>MGHHHHHHMKLTPELTPFVLFTGFEPVQVQQYIKKLYILGGEVAESAQKCTHLIASKVTRTVKFLTAISVVKHIVTPEWLEECFRCQKFIDEQNYILRDAEAEVLFSFSLEESLKRAHVSPLFKAKYFYITPGICPSLSTMKAIVECAGGKVLSKQPSFRKLMEHKQNSSLSEIILISCENDLHLCREYF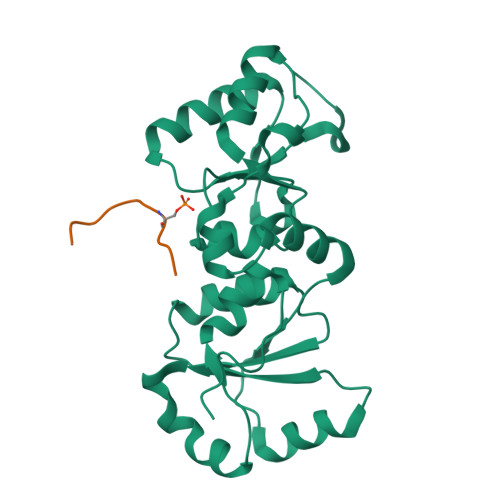ARGIDVHNAEFVLTGVLTQTLDYESYKFN[2x];>KKATQASQEY[2x]>[2x]YKKAGLQRTLVL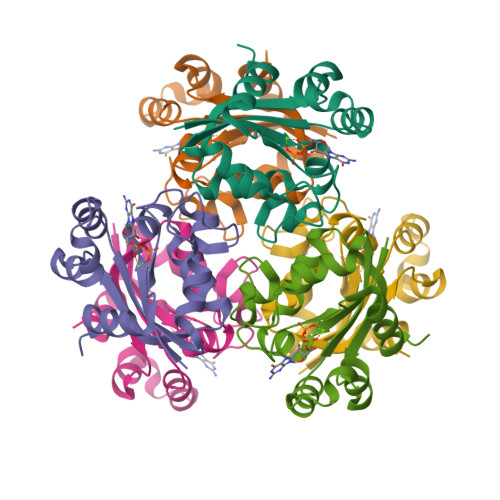IKPDAFERSLVAEIMGRIEKKNFKIVSMKFWSKAPRNLIEQHYKEHSEQSYFNDLCDFMVSGPIISIVYEGTDAISKIRRLQGNTNPLASAPGTIRGDLANDIGENLIHASDSEDSAVDEISIWFPETKMETDN>[6x]GSHMDWKQPELESDEHGKTLRLTLPEGLSGEQKSQWMLTIKA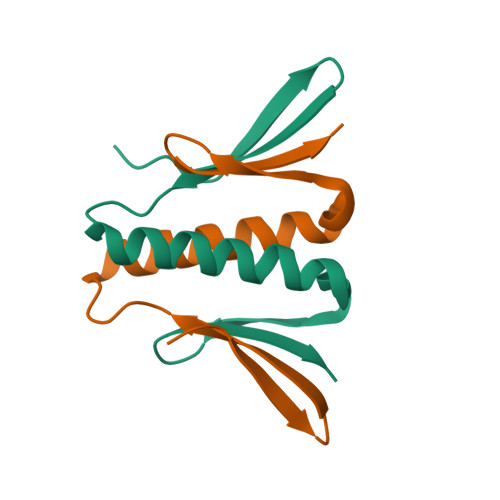VVQSAKHWNLAECTFEASGEGVIIKKRQITPDV>[2x]MTLRSALLALLSSGPLTGYDASQRFGASVGFVWSGSDSQIYPELRKM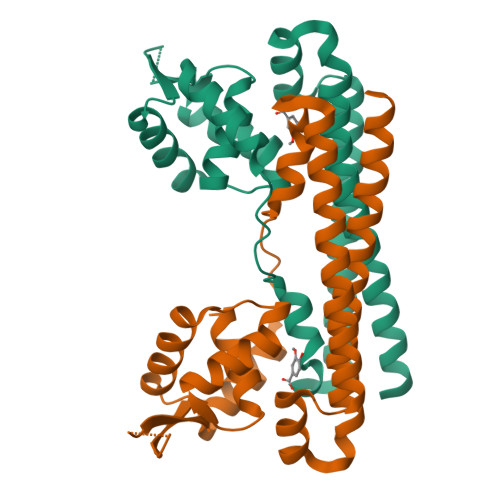EAEELLVGSDVPWGSKGATKTEYALSEKGWEALRKAWYEPVTYGPTRDPARLKAAYFEVGTNGDARRHLRAHIAHFEQQKIQSESMIDELKAKTHPTLARRLERSPKKEHERIVAFKVLAYEGQIARAQAEIEWAEKGLKLLDTL>[4x]MSQVTEQSVRFQTALASIKLIQASAVLDLTEDDFDFLTSNKVWIATDRSRARRCVEACVYGTLDFVGYPRFPAPVEFIAA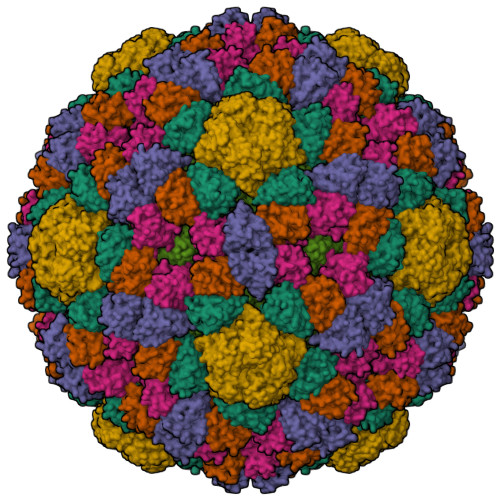VIAYYVHPVNIQTACLIMEGAEFTENIINGVERPVKAAELFAFTLRVRAGNTDVLTDAEENVRQKLRAEGVM;> MEQLTKNQAVATSQEAVQNQNEPQLRDENAHNDKSVHGVLNPTYQAGLRRDAVQPDIEAERKKRDEIEAGKSYCSRRFGGATCDDKSAQIYARFDKNDWRIQPAEFYRFHDAEVNTFGYF;> SNIQTGAERMPHDLSHLGFLAGQIGRLITISTTPVIAGDSFEMDAVGALRLSPLRRGLAIDSTVDIFTFYVPHRHVYGEQWIKFMKDGVNATPLPTVNTTGYIDHAAFLGTINPDTNKIPKHLFQGYLNIYNNYFKAPWMPDRTEANPNELNQDDARYGFRCCHLKNIWTAPLPPETELSRQMTTSTTSIDIMGLQAAYANLHTDQERDYFMQRYRDVISSFGGKTSYDADNRPLLVMRSNLWASGYDVDGTDQTSLGQFSGRVQQTYKHSVPRFFVPEHGTMFTLALVRFPPTATKEIQYLNAKGALTYTDIAGDPVLYGNLPPREISMKDVFRSGDSSKKFKIAEGQWYRYAPSYVSPAYHLLEGFPFIQEPPSGDLQERVLIRHHDYDQCFQSVQLLQWNSQVKFNVTVYRNLPTTRDSIMTS;> MFQTFISRHNSNFFSDKLVLTSVTPASSAPVLQTPKATSSTLYFDSLTVNAGNGGFLHCIQMDTSVNAANQVVSVGADIAFDADPKFFACLVRFESSSVPTTLPTAYDVYPLNGRHDGGYYTVKDCVTIDVLPRTPGNNVYVGFMVWSNFTATKCRGLVSLNQVIKEIICLQPLK(5E)-7-{6-[(1E)-3-HYDROXYOCT-1-ENYL]-2-OXABICYCLO[2.2.1]HEPT-5-YL}HEPT-5-ENOIC 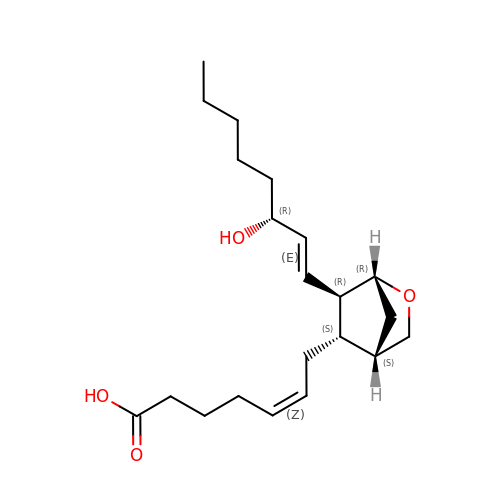ACID | C21 H34 O4 | LQANGKSBLPMBTJ-ZESXDWFFSA-N> CYLSRKLMLDARENLKLLDRMNRLSPHSCLQDRKDFGLPQEMVEGDQLQKDQAFPVLYEMLQQSFNLFYTEHSSAAWDTTLLEQLCTGLQQQLDHLDTCRGQVMGEEDSELGNMDPIVTVKKYFQGIYDYLQEK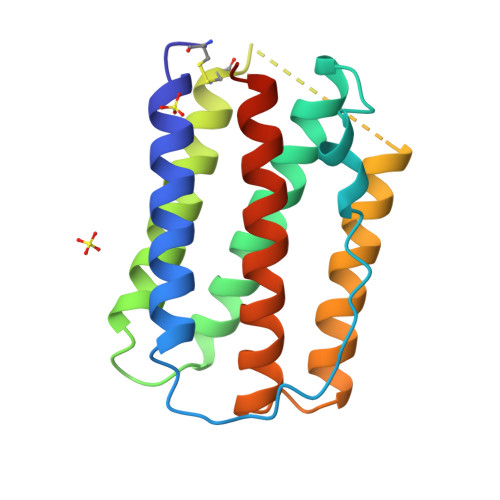GYSDCAWEIVRVEMMRALTVSTTLQKRLTKMGGDLNSP> GHMKHTIDPSSPDFQPIPSFEECFPKSTKEHKEVVHEESGHVLKVPFRRVHLSGGEPAFDNYDTSGPQNVNAHIGLAKLRKEWIDRREKLGTPRYTQMYYAKQGIITEEMLYCATREKLDPEFVRSEVARGRAIIPSNKKHLELEPMIVGRKFLVKVNANIGNSAVASSIEEEVYKVQWATMWGADTIMDLSTGRHIHETREWILRNSAVPVGTVPIYQALEKVDGIAENLNWEVFRETLIEQAEQGVDYFTIHAGVLLRYIPLTAKRLTGIVSRGGSIHAKWCLAYHKENFAYEHWDDILDICNQYDVALSIGDGLRPGSIYDANDTAQFAELLTQGELTRRAWEKDVQVMNEGPGHVPMHKIPENMQKQLEWCNEAPFYTLGPLTTDIAPGYDHITSAIGAANIGALGTALLCYVTPKEHLGLPNRDDVKAGVIAYKIAAHAADLAKQHPHAQAWDDALSKARFEFRWMDQFALSLDPMTAMSFHDETLPADGAKVAHFCSMCGPKFCSMKITEDIRKYAEENGYGSAEEAIRQGMDAMSEEFNIAKKTISGEQHGEVGGEIYLPESYVKAAQK

ThiC, the enzyme discussed here, catalyses the complex rearrangement of aminoimidazole ribonucleotide (AIR) to 4-amino-5-hydroxymethyl-2-methylpyrimidine phosphate (HMP-P) in the thiamin biosynthetic pathways of bacteria and plants 17 and is an example of a non-canonical radical SAM enzyme. The CX2CX4C motif of ThiC varies from the canonical radical SAM motif and is located near the C terminus of the sequence. The homodimeric structure of Caulobacter crescentus ThiC (CcThiC) showed a (β/α)8-barrel fold and suggested that the cluster-binding domain, which was disordered, resides near the C terminus and inserts into the active site of an adjacent protomer through domain swapping. The cluster-binding domain inserts into the active site of an adjacent catalytic domain through domain swapping as previously predicted.

We prepared two different crystal forms of AtThiC, each containing the substrate analogue imidazole ribonucleotide (IRN) and the SAM analogue S-adenosylhomocysteine (SAH), which is also a competitive inhibitor of ThiC21. In the canonical radical SAM enzymes, the SAM amino and carboxylate groups anchor to the differentiated iron in the [4Fe-4S] cluster; however, in ThiC the fourth iron binds to a chloride ion, and the amino and carboxylate groups of SAH anchor to an additional transition metal site. In addition to the amino and carboxylate groups of SAH, the metal is coordinated to two absolutely conserved histidine residues (His426 and His490 in AtThiC and His417 and His481 in CcThiC) and two water molecules. For the crystals grown with addition of ZnSO4, strong fluorescence emission peaks were observed for both Fe and Zn, and a trace-level peak was observed for Ni. The higher level of Zn suggested a bound Zn with the probable site being the metal bound by His426 and His490. Peak heights for a metal at its absorption edge were 60–80 times the root mean square value of the map. The results of the multiwavelength anomalous diffraction experiments using the cluster iron atoms as a reference are shown in Supplementary Table 1 and indicate that in the absence of added ZnSO4 the metal is iron, and that when ZnSO4 is added during crystallization the iron is displaced by zinc. Zinc when added to AtThiC at a 1:1 molar ratio during crystallization largely displaces iron at the additional metal site. In the high-resolution crystal structures of AtThiC containing SAH, the average Fe…S distance from the iron covalently bound to Cys573 is 3.5 Å (range 3.3–3.7 Å) with an average Fe…S-C angle of 165° (range 162°–169°). The three crystal structures determined for AtThiC with bound IRN show that IRN adopts the same binding mode observed in the previously determined structure of CcThiC that lacked a [4Fe-4S] cluster.> SAWRKAGMSYAAYLNVAAQAIRSSLKTELQTASVTNRSQTDAFYTQYKNGTAAS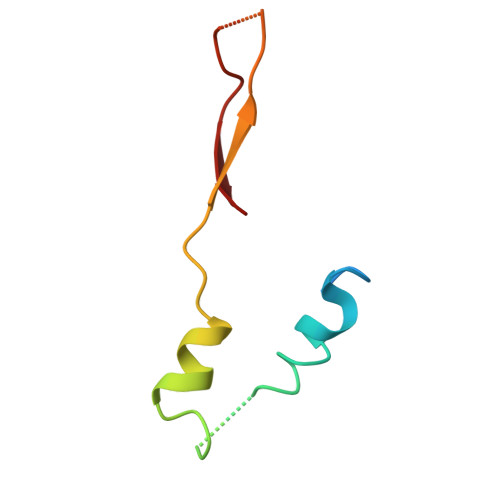EPTPMTK>GSAQEPVKGP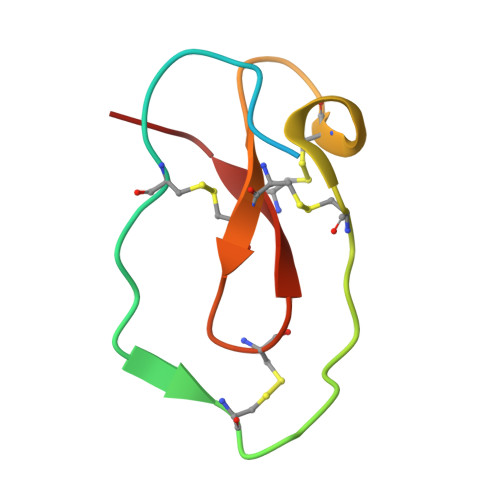VSTKPGSCPIILIRCAMLNPPNRCLKDTDCPGIKKCCEGSCGMACFVPQ[18x]> GPGSGLDSSHVGVRPSPATSQPTTSTGSADLDSILGHMGLPLGNSVLVEEQSTTEFHSILGKLFAAQGIVHNRISDSSADKTRNGDTHVIVLSLNQMFAKELPGIYKGSRKQMKKNLISEEESKVTVQNLNETQRSTPSRYKDLKIAWKYKLADEKRLGSPDRDDIQQNSEYKDYNHQFDITTRLMPAPIASELTFIAPTQPVSTILSQIEQTIKRNDKKLIRIVIPSLLHPAMYPPKMFESSEIIGLMHGVRSLVKKYYERVVLFASISIDIITPPLLVLLRNMFDSVINLEPFNQEMTEFLERVYKSQPGKIQHGLVHILKLPVFTDRGEMRVLKSEWAFKNGRKKFEIEQWGIPVDDAEGSAASEQSHSHSHS;> GPGSMASSSHNPVILLKRILSLTESSPFILCLDSIAQTSYKLIQEFVHQSKSKGNEYPIVYISFETVNKPSYCTQFIDATQMDFVHL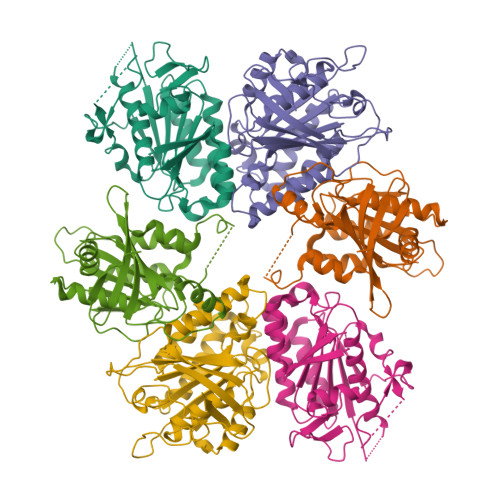VKQIISYLPAATATQAKKHMVIIDSLNYISTEYITRFLSEIASPHCTMVATYHKDIKDENRTVIPDWNNNYPDKLTLLQFMATTIVDIDVVLTGTLDTEEVSELLNEFRIPRGLNNDIFQLRLVNKRKSGRSLEYDFIVNSNTHEYELLSTTKQE;> GPGSMGSVQRQDLVLFSDQSVLPAHFFQDSNSHNLFFITHQSCTQPLWMINALVETHVLGSPSSLNESSSSMLPSSTRSHAVLASFIHEQNYFTNSLNKLKIPSNNYNVLDFLSDFIVNNIHNKPRDKILSDVLAKFSAAIQNNPTDTIVIIEQPELLLSLVSGLTCSELNNKFITPLLRQCKVLIIVSNSDIFNIDEYDASVHSSNLQNFYKSSFIKSMINLNLNPLKTGFAKDVTGSLHVCRGGAPIATSNTSLHVVENEYLYLNEKESTKLFYR>MQIGFNFTLTGTLDMVQQMIKERKIDYVEMLIDNFVHLPPEQIADSFDCPVAFHIMLSKYLERDREALAALGKRLRRFIDVMRPVYVSDHILYFTHNGRSLFHLGEIDYGEYDHVRSKVEQWQDMLGTRLYLENYPSIMDGAWDAPSFYERLSRETGVGVLFDASNAICAQNNTGAPVELWKKIIETTRHFHVAGYGTAFIEPRVKADTSDREMAEDTLDFLSRMRTSFDKPGATITYERDFDIDYESISVDLKRLRDIFPCVEEERH[2x];>[2x]MSLLPTAPVRIDADLYDDLANPARQSLYPRDSRGFIRIDISLRAYWHTLFDTCPRLLELSGPSGGAIFLPFMAWARENN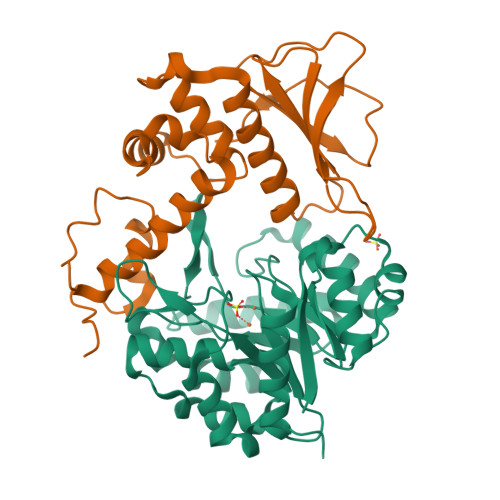LAFDWSFFLWVYVWLQQSEFRERLDEDQLLPVMTASATRWLMIDRDIDACQIVLGSRSLAGAAVVGAKIDSIHCRLEQVQQVAFAAPLPLPDGEFGYFLTPGFEIDHFPGWRPLPR> MIEIKDKQLTGLRFIDLFAGLGGFRLA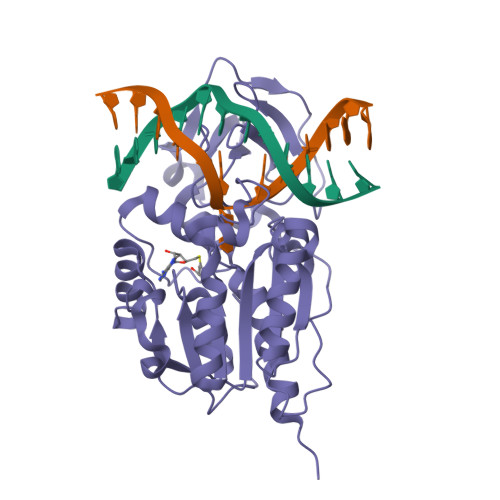LESCGAECVYSNEWDKYAQEVYEMNFGEKPEGDITQVNEKTIPDHDILCAGFPCQAFSISGKQKGFEDSRGTLFFDIARIVREKKPKVVFMENVKNAASHDNGNTLEVVKNTMNELDYSFHAKVLNALDYGIPQKRERIYMICFRNDLNIQNFQFPKPFELNTFVKDLLLPDSEVEHLVIDRKDLVMTNQEIEQTTPKTVRLGIVGKGGQGERIYSTRGIAITLSAYGGGIFAKTGGYLVNGKTRKLHPRECARVMGYPDSYKVHPSTSQAYKQFGNSVVINVLQYIAYNIGSSLNFKPY>MSDSQTLVVKLGTSVLTGGSRRLNRAHIVELVRQCAQLHAAGHRIVIVTSGAIAAGREHLGYPELPATIASKQLLAAVGQSRLIQLWEQLFSIYGIHVGQMLLTRADMEDRERFLNARDTLRALLDNNIVPVINENDAVATAEIKVGDNDNLSALAAILAGADKLLLLTDQKGLYTADPRSNPQAELIKDVYGIDDALRAIAGDSVSGLGTGGMSTKLQAADVACRAGIDTIIAAGSKPGVIGDVMEGISVGTLFHAQATPLENRKRWIFGAPPAGE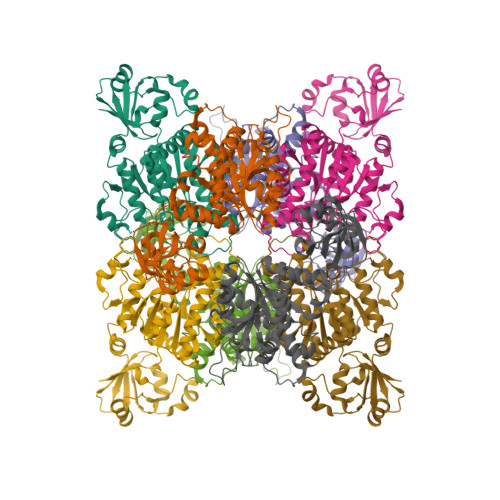ITVDEGATAAILERGSSLLPKGIKSVTGNFSRGEVIRICNLEGRDIAHGVSRYNSDALRRIAGHHSQEIDAILGYEYGPVAVHRDDMITR[8x]> AVNGKGMNPDYKAYLMAPLKKIPEVTNWETFENDLRWAKQNGFYAIMVDFWWGDMEKNGDQQFDFSYAQRFAQSVKNAG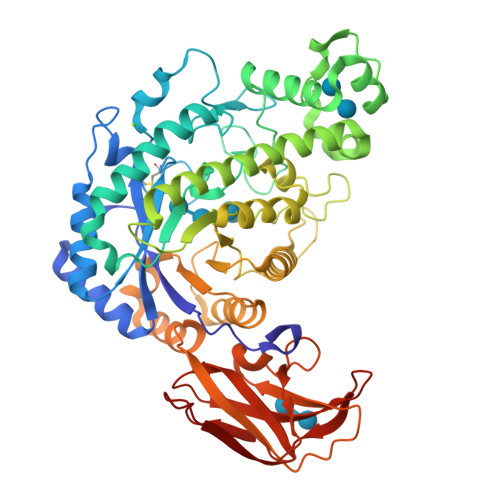MKMIPIISTHQCGGNVGDDCNVPIPSWVWNQKSDDSLYFKSETGTVNKETLNPLASDVIRKEYGELYTAFAAAMKPYKDVIAKIELSGGPAGELRYPSYTTSDGTGYPSRGKFQAYTEFAKSKFRLWVLNKYGSLNEVNKAWGTKLISELAILPPSDGEQFLMNGYLSMYGKDYLEWYQGILENHTKLIGELAHNAFDTTFQVPIGAKIAGVHWQYNNPTIPHGAEKPAGYNDYSHLLDAFKSAKLDVNFTCLEMTDKGSYPEYSMPKTLVQNIATLANEKGIVLNGENALSIGNEEEYKRVAEMAFNYNFAGFTLLRYQDVMYNNSLMGKFKDLLGVTPVMQTIVVKNVPTTIGDTVYITGNRAELGSWDTKQYPIQLYYDSHSNDWRGNVVLPAERNIEFKAFIKSKDGTVKSWQTIQQSWNPVPLKTTSHTSSW> MGSSHHHHHHSQDLEVLFQGPHMAFEKPLRKLTFADLLQATNGFHNDSLIGSGGF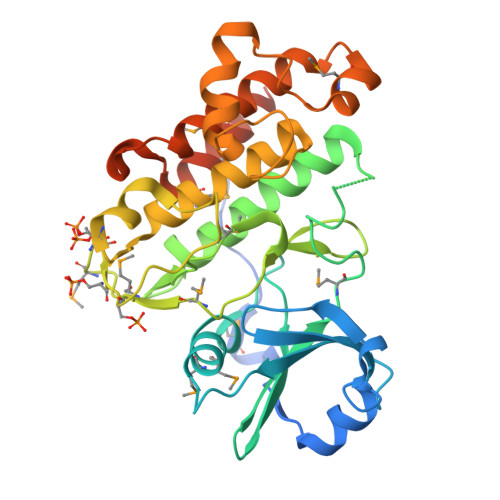GDVYKAILKDGSAVAIKKLIHVSGQGDREFMAEMETIGKIKHRNLVPLLGYCKVGDERLLVYEFMKYGSLEDVLHDPKKAGVKLNWSTRRKIAIGSARGLAFLHHNCSPHIIHRDMKSSNVLLDENLEARVSDFGMARLMSAMDTHLSVSTLAGTPGYVPPEYYQSFRCSTKGDVYSYGVVLLELLTGKRPTDSPDFGDNNLVGWVKQHAKLRISDVFDPELMKEDPALEIELLQHLKVAVACLDDRAWRRPTMVQVMAMFKEIQAGSGIDSQSTIRSIEDGGFST>MTSRIRFLMCPPDHYDVDYVINPWMEGNIHKSSRDRAVEQWQGLYQILKEHAIVDLVTPQKGWPDLVFTANAGLVLGDNVVLSRFLHKERQGEEPYFKEWFEGNGYTVYELPKDLPFEGAGDALLDREGRWLWAGYGFRSELDSHPYLAKWLDIEVLSLRLIDERFYHLDTCFCPLANGYLLYYPGAFDSYSNRLIEMRVAPEKRIAIAEADAVNFACNTVNVESIVIMNKASDALKQSLTGVGFQVLETPLTEFLKAGGAAKCLTLRVTEPVRDEVHANVYVESRIIRIEGHLLDSGLINRALDMIVDTGGSFQVLNFNLGEQRQSTSAAEVKVSAPSHEVMEEIISLLIDLGAVDLPQDERDAKLEPVIQDGVAPDDFYVSTIYPTEVRINGQWIKVENQRMDGAIAITQTPNGLLAQCKILRDLKAGEQVIVDVLGIRTIRKTESREQRNTQEFSFMSGGVSSERRVELVVEQVAWELRKIRDAGGKVVVTAGPVVIHTGGGEHLSRLIREGYVQALLGGNAIAVHDIEQNMMGTSLGVDMKRGVAVRGGHRHHLKVINTIRRHGSIAKGVESGIIRSGVMYECVRN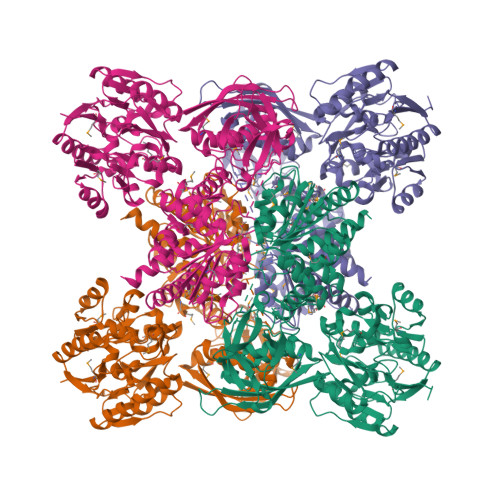QIPFVLAGSIRDDGPLPDTQMDLIKAQEEYAKHLEGAEMILMLSSMLHSIGVGNMTPAGVKMVCVDINPAVVTKLSDRGSIESVGVVTDVGLFLSLLTQQLDKLTSPYVSKVG[2x]> ATGGVKK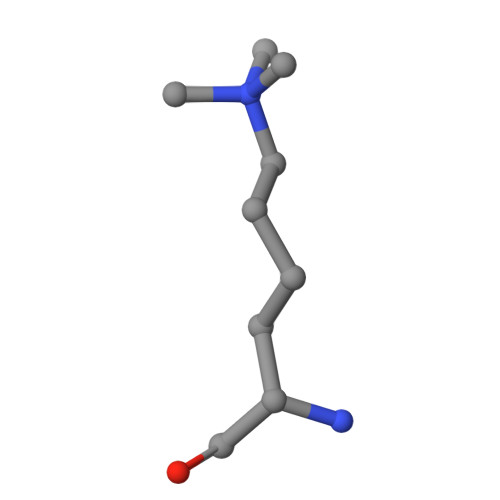PHRY During the replicative cycle of retroviruses, the retrotranscribed viral DNA is integrated into the host chromosome by the viral integrase protein (IN). Retroviral IN consists of three domains: the zinc-binding N-terminal domain (NTD), the catalytic core domain (CCD) and the C-terminal domain (CTD). The central CCD contains an invariant D,D(35)E motif, which forms a catalytic triad with two sites that can coordinate various divalent cations (Mg(II), Mn(II), Zn(II), Cd(II), Ca(II)) although Mg(II) is the likely metal cofactor in vivo. Rous-associated virus type 1 (RAV-1) is a replication-competent alpharetrovirus, member of ASLV subgroup A; the INs of this retrovirus genus are a good model for HIV IN [28].

Herein, we have determined the crystal structure of the CCD of RAV-1 IN to 1.8 Å resolution. Crystals were obtained in the presence of Zn(II) and MES at pH 6.0. They belonged to the hexagonal space group P61 and contained two molecules in the asymmetric unit. The structure contains 271 amino acids in two monomers termed A and B, 186 water molecules, three Zn(II) ions and one MES molecule (left). The present A/B dimer buries three pairs of facing helices (α3A/α5B, α1A/α1B, α3B/α5A) in a new intermolecular interface, which can be obtained from the crystallographic dimer of RSV-A IN CCD by a 15 Å translation of one monomer along the other. Moreover, helices α1 of monomers A and B now run almost parallel to the non-crystallographic two-fold axis and are locked together via a buried Zn(II) that coordinates the imidazole rings of His103A and His103B (left). The area of the buried surface at the new CCD/CCD interface, 740 Å2 per monomer, is similar to that previously observed in RSV-A IN; that is, 750 Å2 per monomer. The novel dimeric interface buries a MES in a canal located between helix α5 of molecule A and helix α3 of molecule B (left). The carboxylate group of Asp64 is situated at the centre of the triad and interacts with Asp121 through a Zn(II) ion from the crystallization solution.

>GSGRGLGPLQIWQTDFTLEPRMAPRSWLAVTVDTASSAIVVTQHGRVTSVAAQHHWATAIAVLGRPKAIKTDNGSCFTSKSTREWLARWGIAHTTGIPGNSQGQAMVERANRLLKDKIRVLAEGDGFMKRIPASKQGELLAKAMYALNHF[2x]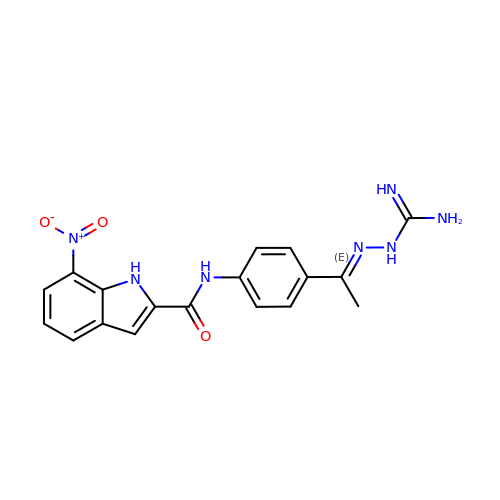N-[4-[(E)-N-carbamimidamido-C-methyl-carbonimidoyl]phenyl]-7-nitro-1H-indole-2-carboxamide | C18 H17 N7 O3 | ZKHRFTLMLVMQMS-AUEPDCJTSA-N> MRKRELLNEARALVPEGSGWLEAYTRNISPRQLTWRLGKRDSLAAMTEGWQLYQGKFDTVAMAALLRRLRHAQLQDPGFDPLAAQRLLDDLVPRLRSVGLRFGKLRDITAYLHALAKLRSPAPSASSSAASPRAGAAAASLLTQPDALVLDLAVFATRNRTELLHASPQRLATLLWALMRLLPPQLYGSEQLQV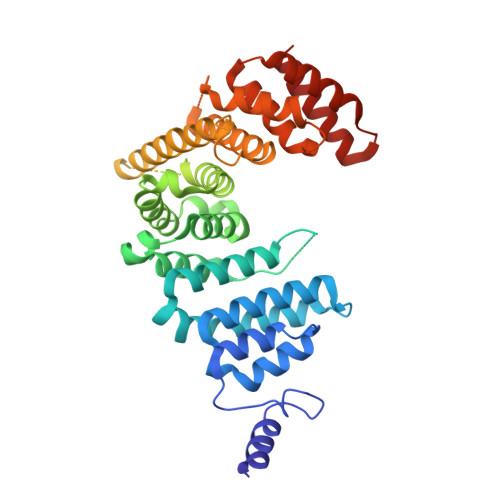VLDRMALASLGRLQNFAPLDLRWAALAFATFGPHGPSSKATATTTAAAAGTRAAAGAGSGPALPEWPRVVRGEAAAAATAGAQGAEDVTARRQSRNARVIKALCDELAARSGNLALPQPEPRDLALAAHALGLVAAASSSAGGAVAPPALLVKAAGVAARSLPALSGEEAVGLVETLAVWGLRQPALLEALRDAAGRWGEGEQAEALRGRLQAAYTRLGVEL> MMLLSKGRPAMRSRILTSLMLSLAVAPTAYAQQENEEEQDTGGEMGGAEVMDEAPDSAPPTSVAMPPGAPRGRESAPGEVHSVESGDTLWDLSQRYLGSPWYWPKVWSYNPEIANPHWIYPGNQVRFFAAGEEVPTQVTEMVVDEGDVTAPMEMTSNDQVIVTGKIGVDLANSVPVTTQ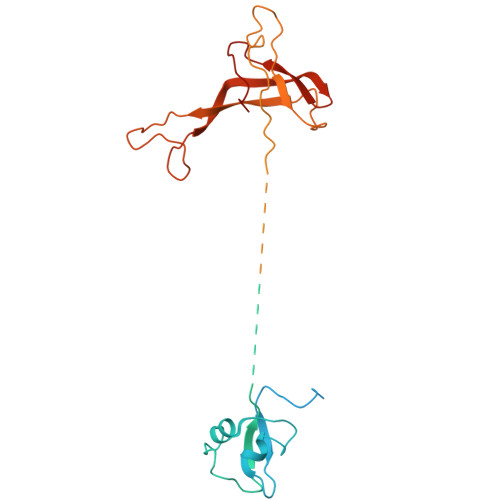GFVTQRELDEAGRIEGSPSNAVMLSFPDSVYVRFKRKGDVKVGDRYVVYHTTQAVKHPVTGRPLGFLTDFVGTLRVQRVGDGIVTAQIMDTWDGIERGDLVGPVGERLTERVAPKPNAKQVDGTVITALVPYLTVLGENHSIVVDKGSADGVELGNTFNILRKGDPSRHVLGHDVRKPSKEEQSFPWRSIGACMVTEVKERTSNCLMTRSLEELVPGDRAHMSAGASPSASR>SMKDIWHPGERCLAP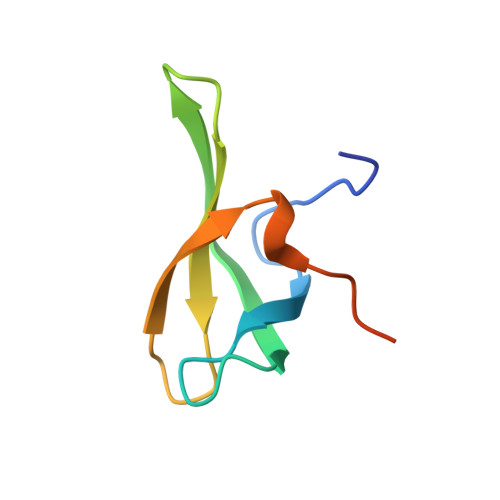SPDNGKLCEASIKSITVDENGKSFAVVLYADFQERKIPLKQLQEVKFVKDCPRN[2x]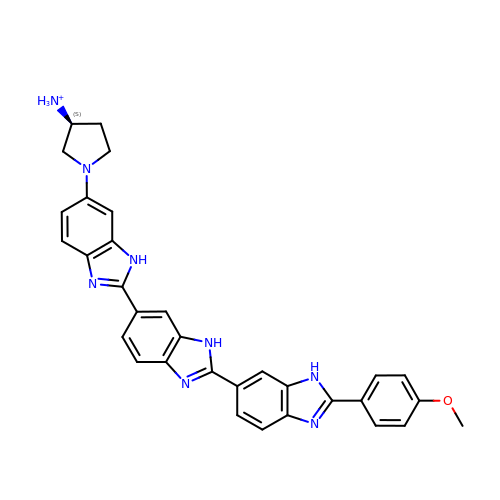2''-(4-METHOXYPHENYL)-5-(3-AMINO-1-PYRROLIDINYL)-2,5',2',5''-TRI-BENZIMIDAZOLE | C32 H29 N8 O | MEDNUDGNJOXVKL-NRFANRHFSA-O> EYEIIETIGNG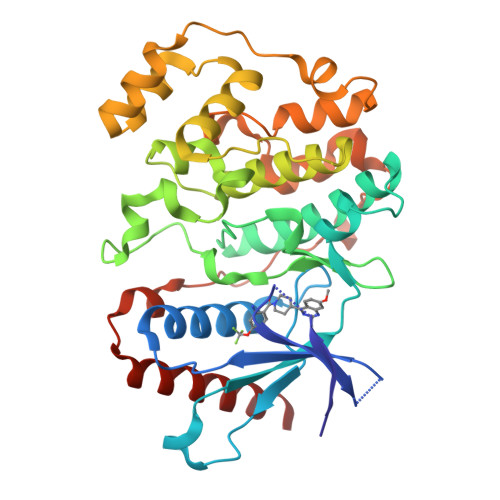AYGVVSSARRRLTGQQVAIKKIPNAFDVVTNAKRTLRELKILKHFKHDNIIAIKDILRPTVPYGEFKSVYVVLDLMESDLHQIIHSSQPLTLEHVRYFLYQLLRGLKYMHSAQVIHRDLKPSNLLVNENCELKIGDFGMARGLCTSPAEHQYFMTEYVATRWYRAPELMLSLHEYTQAIDLWSVGCIFGEMLARRQLFPGKNYVHQLQLIMMVLGTPSPAVIQAVGAERVRAYIQSLPPRQPVPWETVYPGADRQALSLLGRMLRFEPSARISAAAALRHPFLAKYHDPDDEPDCAPPFDFAFDREALTRERIKEAIVAEIEDFHARRE>MGSSHHHHHHSSGRENLYFQGMNTLQLINKNHPLKKNQEPPHLVLAPFSDHDVYLQPEVAKQWERLVRATGLEKDIRLVSGYRTEKEQRRLWEYSLKENGLAYTKQFVALPGCSEHQIGLAIDVGLKKQEDDDLICPHFRDSAAADLFMQQMMNYGFILRYPEDKQEITGISYE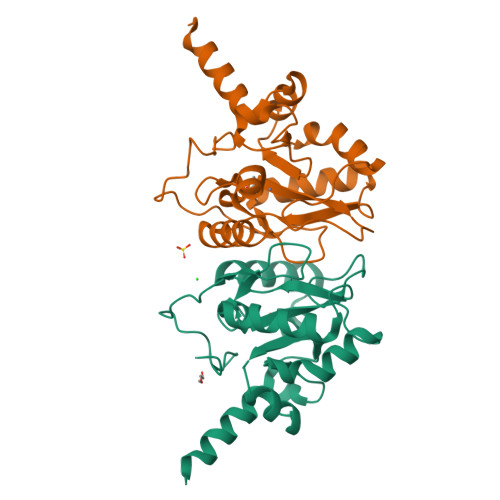PWHFRYVGLPHSQVITAQKWTLEEYHDYLAQTVRQFA[2x]>AELDGDQMISHRELWAKIANSINDINEQYLKVYEHAVSSYTQMYQDFSAVLSSLAGWISPGGNDGNSVKLQVNSLKKALEELKEKYKDKPLYPANNTVSQEQANKWLTELGGTIGKVSQKNGGYVVSINMTPIDNMLKSLDNLGGNGEVV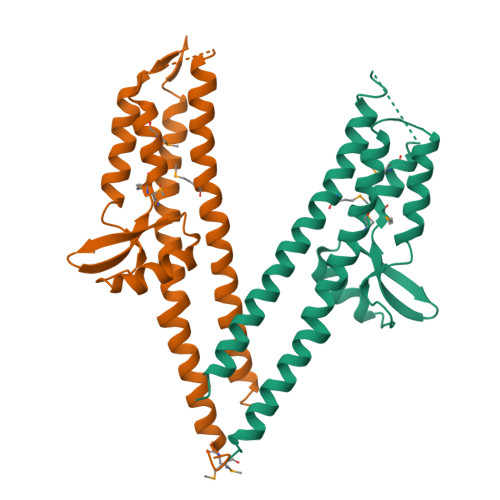LDNAKYQAWNAGFSAEDETMKNNLQTLVQKYSNANSIFDNLVKVLSSTISSCTDTDKLFLHF[2x]TACAN, originally identified in a proteomics screen and called TMEM120A, was categorized as a nuclear envelope protein (NET29) that participates in lipid metabolism. TACAN is an α-helical TM protein that forms a symmetric dimer. Each protomer consists of six TM helices (S1–S6), which form a barrel surrounding a tunnel open to the cytoplasm. The TACAN protomer is related in three-dimensional structure to a fatty acid elongase, ELOVL7.

To determine the identity of the small molecule implied by the broken density in the tunnel of TACAN, we determined the structure of TACAN with His196 and His197 mutated to alanine at 2.8 Å resolution. Our rationale was that if the His residues are catalytically important – by analogy to ELOVL7 – then their mutation might influence the occupancy of a potential cofactor. The map showed clearer density consistent with a coenzyme A molecule (CoASH). Native mass spectrometry (nMS) was used to confirm the identity as CoASH. The purified TACANH196A H197A sample contains a mixture of the 83,237 Da, +767 Da, and +1535 Da mass species, corresponding to an apo form, one and two CoASH bound forms, respectively. After incubation with CoASH, some fraction of the apo form shifts to one and two CoASH bound forms. Additionally, the +767 Da and +1535 Da species are replaced by +795 Da and +1591 Da or +811 Da and +1622 Da species after incubation with the two CoASH analogues S-ethyl-CoA or Acetyl-CoA, corresponding to the CoASH analogue bound forms. In the purified TACANWT sample, the apo form is dominant and incubation with S-ethyl-CoA shifts it to one and two analogue bound forms. Together, these data are consistent with our cryo-EM results and indicate that TACAN is co-purified with endogenous coenzyme A. ELOVL7 showed significant activity, while neither the wild-type nor His196Ala His197Ala mutant of TACAN showed any activity.

>[2x]MQSPPPDPLGDCLRNWEDLQQDFQGIQETHRLYRLKLEELTKLQANCTNSITRQKKRLQELALVLKKCRPSLPSESMEAAQELENQMKERQGLFFDMEAYLPKKNGLYLSLVLGNVNVTLLSKQAKFAYKDEYEKFKLYLTIILIVISFTCRFLLNSRVTDAAFNFLLVWYYCTLTIRESILINNGSRIKGWWVFAAYVSTFLSGVMLTWPDGLMYQKFRNQFLSFSMYQSFVQFLQYYYQSGCLYRLRALGERHTMDLTVEGFQSWMWRGLTFLLPFLFFGHFWQLFNALTLFNLARDPECKEWQVLMCGFPFLLLFLGNFFTTLRVVHQKFHSQQHGNKKD>SNATEELTTVRDACARTLENTARTLHLGASGTEFVAAFRAMTDHWGAARPHDLPLSDVSPDGSPVEYAVDLGGLAPALQFAMEPLTAGVPARDPLAARAIMPLLAGRYGADATRWSALADRLLPDDAHGPHVSMYGAEVRAGAPIRFKAWFYLNVTGPDGAFNLLYSALERMGTTHLWPVVQAHVHRAGEDVPFLLSLDLSDDPAARVKVYFRHFAADVEEVAAVLKAYPGFEPGEVRAFCKVMMGGRRRFSDQPAVTCVSLLDAQTFDRTAATLYVPLWTYAEHDGEVRQRVHRTLAAWPEALYRYDSVLAGIAHRGLDAGTGIHNYISWQPGRTRPRMKVYLSPEMHDVTPPPLGVSQQHHLSGQTTA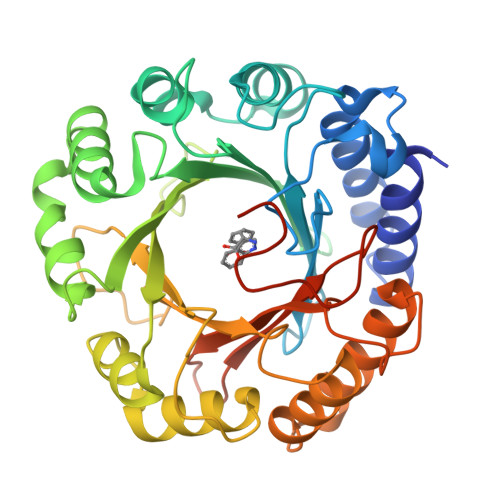RGRTE[3x]> QECTKFKVSSCRECIESGPGCTWCQKLNFTGPGDPDSIRCDTRPQLLMRGCAADDI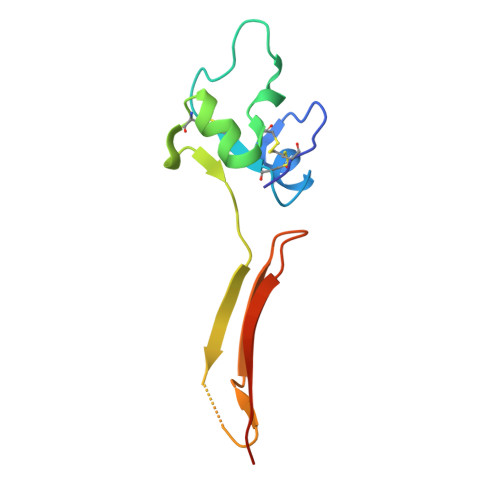MDPTSLAETQEDHNGGQKQLSPQKVTLYLRPGQAAAFNVTFRRAKGY Fortunately, the RT/RH domains of HBV Pol exhibit weak sequence homology with human immunodeficiency virus type-1 (HIV-1) RT. In particular, a consensus sequence present across multiple regions (i.e., Motifs A, B, C and D) that creates a dNTP-binding site (N-site) for HBV/HIV-1 RT is significantly conserved. We therefore newly generated HBV RT-mimicking HIV-1 RT mutants by substituting unconserved N-site residues with corresponding amino acids in the HBV RT sequence. Here, we report the acquisition of 3TC/ETV resistance using HIV-1 with three HBV-associated amino acid substitutions (F115Y/Y116F/Q151M) in the RT N-site.

Importantly, we found that additional mutations F160M/M184V in RT rendered HIV3MB virtually fully resistant to both 3TC and ETV. To experimentally explore the structural effects of the Met184 substitution with Val/Ile, we also determined the HIV-1 RT3MB/F160M/M184V:DNA:3TC-TP ternary complex structure at a resolution of 2.57 Å. We found that two RT molecules in the asymmetric unit were in different conformations: one in a closed conformation identical to other RT3MB ternary complexes, whereas the other molecule was in an open conformation reported previously for the RTQ151M:DNA binary complex structure. Despite the difference in RT conformations, a well-defined electron density observed at both RT N-sites enabled us to build the atomic model for the cytosine base and oxathiolane moiety of 3TC-TP. However, electron density for the triphosphate and Mg2+ was quite ambiguous and we were unable to construct the model, indicating loose binding of 3TC-TP to RT3MB/F160M/M184V. The structure revealed that oxathiolane deviates from that in the RT3MB ternary complex by a maximum deviation of ~1 Å. The sulfur atom is located at the gap between Asp185 side-chain carboxyl and the 3′-end nucleotide ribose of the primer, with a distance between the sulfur atom of 3TC-TP and Cγ1 of Val184 in chains A and C of 4.37 Å (chain A) and 4.06 Å (chain C), respectively. The structural superimposition of RT3MB/F160M/M184V and RT3MB also showed that both the methylene C44 of ETV-TP and the sulfur of 3TC-TP are located 2.8–3.0 Å from Cγ1 of Val184, indicating a severe steric clash. Interestingly, the Cγ1 and Cγ2 of Val184 coincides with Cγ of Met184 in normal and backward conformations, respectively, indicating that the χ1 angle of the residue 184 side-chain is significantly restricted. The structure of HIV-1 RT3MB/F160M/M184V:DNA in complex with 3TC-TP also showed that bound 3TC-TP deviated from the tight binding position observed in RT3MB with disordered triphosphate moiety, indicating a steric clash evasion with Val184 Cγ1.

>[2x]MVPISPIETVPVKLKPGMDGPKVKQWPLTEEKIKALVEICTEMEKEGKISKIGPENPYNTPVFAIKKKDSTKWRKLVDFRELNKRTQDFWEVQLGIPHPAGLKQKKSVTVLDVGDAFYSVPLDKDFRKYTAFTIPSINNETPGIRYQYNVLPMGWKGSPAIMQSSMTKILEPFRKQNPDIVIYQYVDDLYVGSDLEIGQHRTKIEELRQHLLRWGFTTPDKKHQKEPPFLWMGYELHPDKWTVQPIVLPEKDSWTVNDIQKLVGKLNWASQIYAGIKVRQLSKLLRGTKALTEVVPLTEEAELELAENREILKEPVHGVYYDPSKDLIAEIQKQGQGQWTYQIYQEPFKNLKTGKYARMKGAHTNDVKQLTEAVQKIATESIVIWGKTPKFKLPIQKETWEAWWTEYWQATWIPEWEFVNTPPLVKLWYQLEKEPIIGAETFYVDGAANRETKLGKAGYVTDRGRQKVVPLTDTTNQKTELQAIHLALQDSGLEVNIVTDSQYALGIIQAQPDKSESELVSQIIEQLIKKEKVYLAWVPAHKGIGGNEQVDKLVSAG;>[2x]MAHHHHHHALEVLFQGPISPIETVPVKLKPGMDGPKVKQWPLTEEKIKALVEICTEMEKEGKISKIGPENPYNTPVFAIKKKDSTKWRKLVDFRELNKRTQDFWEVQLGIPHPAGLKQKKSVTVLDVGDAYFSVPLDKDFRKYTAFTIPSINNETPGIRYQYNVLPQGWKGSPAIFQSSMTKILEPFRKQNPDIVIYQYMDDLYVGSDLEIGQHRTKIEELRQHLLRWGFTTPDKKHQKEPPFLWMGYELHPDKWTVQPIVLPEKDSWTVNDIQKLVGKLNWASQIYAGIKVRQLSKLLRGTKALTEVVPLTEEAELELAENREILKEPVHGVYYDPSKDLIAEIQKQGQGQWTYQIYQEPFKNLKTGKYARMKGAHTNDVKQLTEAVQKIATESIVIWGKTPKFKLPIQKETWEAWWTEYWQATWIPEWEFVNTPPLVKLWYQ>[2x]MSHKAWQNAHAMYENDACAKALGIDIISMDEGFAVVTMTVTAQMLNGHQSCHGGQLFSLADTAFAYACNSQGLAAVASACTIDFLRPGFAGDTLTATAQVRHQGKQTGVYDIEIVN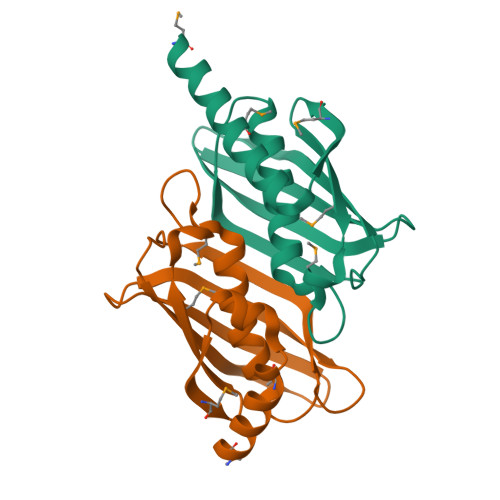QQQKTVALFRGKSHRIGGTITGEA>MALAKRIDAALILKDGRVVKGSNFENLRDSGDPVELGKFYSEIGIDELSFWDITASVEKRKTMLELVEKVAEQIDIPITVGGGIYDFETASELILRGADKVEINTAAVENPSLITQIAQTFGSQAVVVYIAAKRVDGEFMVFTYSGTKNTGILLRDWVVEVEKRGAGEIVLGSIDRLGTKSGYDTEMIRFVRPLTTLPIIAHRGAGKTEHFLEAFLAGADAAKADSVFHSREIDVRELKEYLKKHGVNVRLEGLGSLEHHHHHH[12x]

Computational design of KE07 involved construction of a theozyme to catalyze the chemical reaction, which was then grafted into the scaffold of imidazole glycerol phosphate synthase (HisF) from Thermotoga maritima. Catalytically essential residues from the initial design include a base (Glu101) that facilitates C−H bond cleavage, an H-bond donor (Lys222) to stabilize the phenoxide intermediate, and a π-stacking residue (Trp50), which was designed to stabilize the transition state and favor substrate binding through interactions with the aromatic ring of the substrate. This initial KE07 design (Round 1; R1) catalyzes the cleavage of 5-nitrobenzisoxazole, with 103-fold rate acceleration over the noncatalyzed reaction and a turnover rate (kcat) of 0.018 s−1.

The mutations in R7 and R7-2 (Phe77Ile, Phe229Ser, Ile102Phe) result in further optimization of activation energy. However, the most striking result came from a crystal structure with 12 different KE07 molecules within the asymmetric unit‚ into which substrate was soaked. In this structure, we observe both configuration A (three subunits) and B (one subunit), as well as two additional configurations (hereafter denoted configurations C and D). In configuration C, Trp50 is rotated back to a similar position as the designed conformation, except it is rotated such that the NH of the indole ring can hydrogen bond to the catalytic Glu101. The four subunits in configuration C all had product bound, and were the only chains where product was observed. Four subunits were observed to adopt configuration D, in which Trp50 was disordered in-between the well-defined configurations, supporting the idea that these conformational substates exist in equilibrium. However, in later generations (R7 and R7-2) evidence for turnover was only observed with configuration C. By R7 and R7-2, configuration C (which was the only state we saw associated with product in the crystal structures) becomes the dominant substate sampled, with configurations A and B sampled only rarely.>XGELAQALKELAKALKELAWALKELAQALKGX[3x]

CCs are quaternary structures comprising two or more α-helices supercoiled around each other with cyclic (Cn) or dihedral (Dn) symmetry. Here, we describe variants with all combinations of the aliphatic residues, Ile, Leu and Val, at a and d to give four classes of peptide: the ββ class, with a and d = Ile or Val; Lβ, a = Leu and d = Ile or Val; βL, a = Ile or Val and d = Leu; and LL, a = d = Leu. Peptides are named systematically appending the one-letter code for the amino acids at the a and d sites to “CC-Type2-“; e.g., CC-Hept becomes CC-Type2-LI. In summary, solution-phase data and X-ray crystal structures demonstrate conclusively that different classes of Type-2 coiled-coil (CC) peptides—i.e., based on abcdefg repeats with predominantly hydrophobic residues at a, d, e and g—adopt a range of distinct states.

By contrast, those of the βL class and peptide CC-Type2-LL showed weak or non-specific binding of DPH. And LL sequences form collapsed structures. Surprisingly, the X-ray crystal structure of CC-Type2-LL-L17E overlaid almost perfectly with that for the parent CC-Type2-LL; i.e., all six Glu-17 side chains are completely buried within the core of the assembly. However, the cognate structure for each sequence did not always have the lowest score, as apparent from the off-diagonal white and blue points. This occurs for all of the LL-based sequences and those βL sequences observed to form collapsed structures. For these, we propose that the collapsed states are adopted as they lead to more hydrophobic burial and contacts.>MGSSHHHHHHSSGLVPRGSVPRVFVAGGAGFIGSHYVRELVAGAYAGWQGCEVTVLDSLTYAGNLANLAGVRDAVTFVRGDICDGRLLAEVLPGHDVVLNFAAETHVDRSIADSAEFLRTNVQGVQSLMQACLTAGVPTIVQVSTDEVYGSIEAGSWSEDAPLAPNSPYAAAKAGGDLIALAYARTYGLPVRITRCGNNYGPYQFPEKVIPLFLTRLMDGRSVPLYGDGRNVRDWIHVADHCRGIQTVVERGASGEVYHIAGTAELTNLELTQHLLDAVGGSWDAVERVPDRKGHDRRYSLSDAKLRALGYAPRVPFADGLAETVAWYRANRHWWEPLRKQLDAVPHD[2x]

Herein we identify a new glucuronic acid decarboxylase from Micromonospora belonging to the superfamily of short-chain dehydrogenase/reductase enzymes, EvdS6. Biochemical characterization demonstrated that EvdS6 is an NAD+-dependent bifunctional enzyme that produces a mixture of two products, differing in the sugar C-4 oxidation state. At a global level, EvdS6 displays the SDR enzyme architecture and is a dimer with a buried surface area of 2371 Å2 and 2362 Å2 in ligand-free and nucleotide diphosphate-bound states, respectively. In line with the SDR architecture, each protomer consists of two domains: the N-terminal domain consisting of residues V1-Y181 and V219-A242 and the C-terminal domain between residues G182-H218 and G243-L323.

Structures of EvdS6 were determined, with copurified NAD+, either without additional ligand or with nucleotide diphosphate. In these EvdS6 crystal structures, the enzyme crystallized with two protein chains in the asymmetric unit. In the ligand-free structure, no traceable electron density for residues R273, K274, or G275 or the sidechain of H276 was observed in one of the subunits. One possibility is related to a flexible active site loop that gains order upon substrate binding.> MGKKIHARDLREQRKTDRTEKFADQNKKREAERAVPKKDAAVSVKSVSSVSSKKDNVTKSMAKAAGVKSVFAVGNTVYMTSFGRGNDAVLEQKIVDTSHEPLNIDDPAYQLNVVTMNGYSVTGHRGETVSAVTDNPLRRFNGRKKDEPEQSVPTDMLCLKPTLEKKFFGKEFDDNIHIQLIYNILDIEKILAVYSTNAIYALNNMSADENIENSDFFMKRTTDETFDDFEKKKESTNSREKADFDAFEKFIGNYRLAYFADAFYVNKKNPKGKAKNVLREDKELYSVLTLIGKLAHWCVASEEGRAEFWLYKLDELKDDFKNVLDVVYNRPVEEINNRFIENNKVNIQILGSVYKNTDIAELVRSYYEFLITKKYKNMGFSIKKLRESMLEGKGYADKEYDSVRNKLYQMTDFILYTGYINEDSDRADDLVNTLRSSLKEDDKTTVYCKEADYLWKKYRESIREVADALDGDNIKKLSKSNIEIQEDKLRKCFISYADSVSEFTKLIYLLTRFLSGKEINDLVTTLINKFDNIRSFLEIMDELGLDRTFTAEYSFFEGSTKYLAELVELNSFVKSCSFDINAKRTMYRDALDILGIESDKTEEDIEKMIDNILQIDANGDKKLKKNNGLRNFIASNVIDSNRFKYLVRYGNPKKIRETAKCKPAVRFVLNEIPDAQIERYYEACCPKNTALCSANKRREKLADMIAEIKFENFSDAGNYQKANVTSRTSEAEIKRKNQAIIRLYLT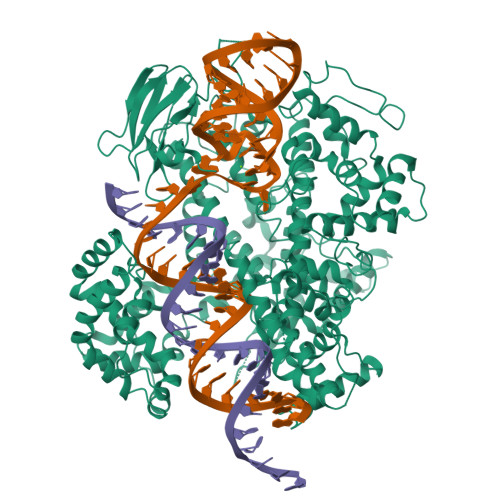VMYIMLKNLVNVNARYVIAFHCVERDTKLYAESGLEVGNIEKNKTNLTMAVMGVKLENGIIKTEFDKSFAENAANRYLRNARWYKLILDNLKKSERAVVNEFANTVCALNAIRNININIKEIKEVENYFALYHYLIQKHLENRFADKKVERDTGDFISKLEEHKTYCKDFVKAYCTPFGYNLVRYKNLTIDGLFDKNYPGKDDSDEQK>[2x]MLTNNISKSKLSGKNIGIYFGTFAPLHTGHQQQIYKCASLNDGVLLVVSGYDNDRGAQIGLPLEKRFRYLREAFNDEENIKVSMLNENDLPEMPNGWDEWANRLFELI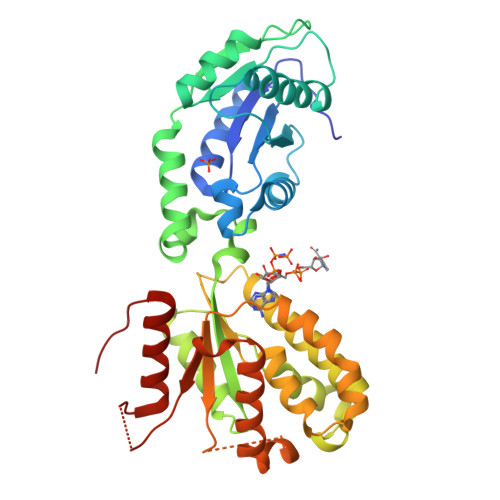HHNTLENDLSVTFYVGELEYAAELKKRFPADGNQYAVEIADRHDISLSATQIRENPQEHWTHINRVFRRHFSKVVTVMGSASTGKTTLVRRLARSINAPFSEEYAREYEEAFNIDDDELKMDDYARMITGQYDANSREVNSPANQGIVFLDTDAIVTRVYAKLYLPKEDFEQLEPLFRKTIADERMDLILVIPPITEYIDDGFRHMEWEESRHEFHEELMRQLAEFGLLDKVVILDDEGDHRDQEGYLTRYHHAIDAVHEYTGVKIERLSY> QFAKPEDAVKYRQSALTLMASHFGRMTPVVKGQAPYDAVQIKANVEVLKTLSALPWAAFGPGTEGGDA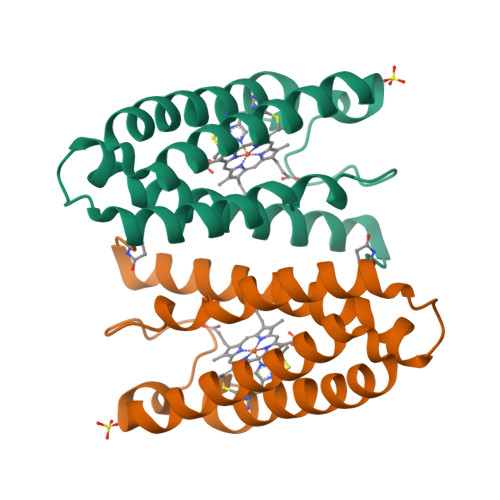RPEIWSDAASFKQKQQAFQDNIVKLSAAADAGDLDKLRAAFGDVGASCKACHDAYRKKK Hunter syndrome, also known as Mucopolysaccharidosis type II (MPS II, OMIM 309900), is an X-linked lysosomal storage disease caused by genetic deficiency of the enzyme iduronate-2-sulfatase (IDS, EC 3.1.6.13), required for the step-wise degradation and recycling of complex glycosaminoglycans (GAGs). IDS belongs to the sulfatase family of enzymes and catalyses hydrolysis of the C2-sulfate ester bond at the non-reducing end of 2-O-sulfo-α-L-iduronic acid residues in dermatan sulfate and heparan sulfate. Despite low sequence identity, the overall fold and domain organization bears a striking core resemblance to other human sulfatases. IDS adopts a compact, globular α/β sandwich fold, comprising residues 34–550.

Here we report the X-ray crystal structure of human IDS with a sulfate ion bound covalently in the active site. The crystal structure of IDS was refined at 2.3 Å resolution. The enzyme is monomeric with a single-polypeptide chain in the asymmetric unit. Lack of interpretable electron density prevented the modelling of one loop region (residues 444–453). Continuous electron densities were observed adjacent to all asparagine residues involved in N-linked glycosylation, and at least one N-acetylglucosamine moiety linked to the nitrogen of the asparagine side chain was built at each predicted site. FGly functions catalytically as an aldehyde hydrate (FGly aldehyde-hydrate, FGH) with two geminal hydroxyl groups; here we observe what we have interpreted as a covalent sulfate-ester intermediate (FGly sulfate, FGS) in the IDS active site, which could originate from natural substrate encountered in cells during expression. The covalent linkage is unambiguous, with a distance of 1.5 Å between the sulfur atom and the FGS ester oxygen. Extra electron density for a metal ion was observed next to the modified FGS residue. This was modelled as Ca2+, coordinated by one nitrogen and five oxygen atoms with approximate octahedral geometry: one oxygen each from the side chains of D45, D46 and D334; two sulfate oxygens from FGS84 and one nitrogen from the side chain of H335. Side chains of conserved H138 and H229 likely play important roles in catalysis, making direct contacts with the free geminal hydroxyl of FGS and a sulfate oxygen (OS3) of FGS, respectively. The arrangement of the IDS active site is compatible with the consensus TE mechanism, hence we propose a similar mechanism for IDS in which FGH84 performs an SN2 nucleophilic attack on the sulfur atom to generate the covalent FGS adduct, followed by elimination of bound sulfate and rehydration of the resultant FGly aldehyde.

> SETQANSTTDALNVLLIIVDDLRPSLGCYGDKLVRSPNIDQLASHSLLFQNAFAQQAVAAPSRVSFLTGRRPDTTRLYDFNSYWRVHAGNFSTIPQYFKENGYVTMSVGKVFHPGISSNHTDDSPYSWSFPPYHPSSEKYENTKTCRGPDGELHANLLCPVDVLDVPEGTLPDKQSTEQAIQLLEKMKTSASPFFLAVGYHKPHIPFRYPKEFQKLYPLENITLAPDPEVPDGLPPVAYNPWMDIRQREDVQALNISVPYGPIPVDFQRKIRQSYFASVSYLDTQVGRLLSALDDLQLANSTIIAFTSDHGWALGEHGEWAKYSNFDVATHVPLIFYVPGRTASLPEAGEKLFPYLDPFDSASQLMEPGRQSMDLVELVSLFPTLAGLAGLQVPPRCPVPSFHVELCREGKNLLKHFRFRDLEEDPYLPGNPRELIAYSQYPRPSDIPQWNSDKPSLKDIKIMGYSIRTIDYRYTVWVGFNPDEFLANFSDIHAGELYFVDSDPLQDHNMYNDSQGGDLFQLLMP>MNHKVHHHHHHIEGRHMYSPDRRAALNSVANMVSDNADKDLRYGGLVHDLLADSGKATPNSDAMEDAFGTWTYQELLNHSQAFSAWLDGKGVARGERIVVQLPNIRQTVAVFYGACRRGVVFVPLNPGMKPFHLRSVIADADPRLVIAEDETAADRLRDVTDLPVYSIDSLWADVERLRDAGAG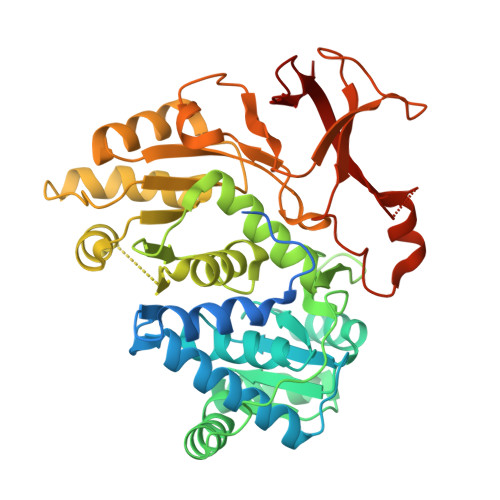AEAVEVSPEDLAVLIYTSGSTAAPKAVACPHQQIVFAASSINAVLGYHAEDIVFCRMSVSWDFGLYKVLISTLTGAKLVLAGGEPDIALVKSLRESGATMMPIVPSLASMLTTLIRRDPEGAPTLRMFTNSAAALPQVTIDALRSAFPGAQVVRMYGQTECKRISIMPPHLEHERPDSVGLPLPGTTIEILDEDGTLLPPGEPGEITVTGPHVMAGYWRAPEITARAYRRDETTGAMRLHTGDYGHLDEDGFLYFGGR[2x]> MAIRNFVFKISNQIQNLAAKRSLAYLNQIDSQSVPSRATINMKDQVTQMQREIDNMANVIRAQIPDEDRAEFEILKK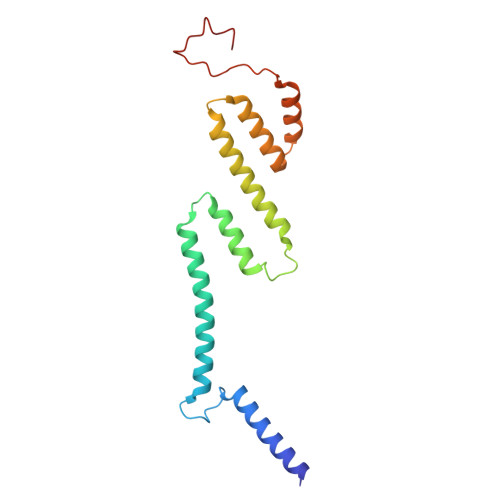YYVTGQHDSLVDPQDVLLQLDRIQVLKNLKMIELNEEAYDPELVRLEKLKARVLLEEEGALLEYAHFISKRPYNKPYEKWGVSEEHVKQQILG>[2x]GSMTRFFTKLDADKSY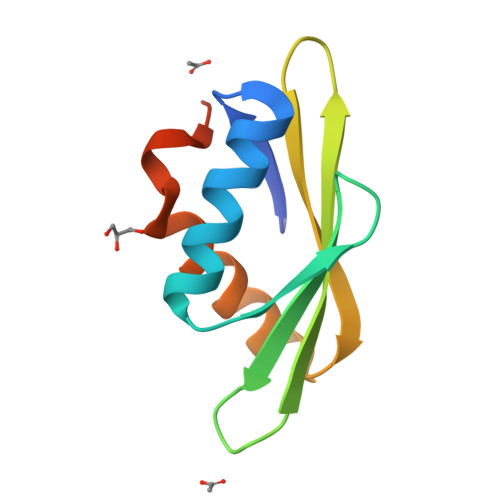QCLKETCEKLGYQWKKSCMNQVTISTTDRRNNKLIFKVNLLEMDDKILVDFRLSKGDGLEFKRHFLKIKGKLIDIVSSQKVWLPAT>[2x]MTYTTRQIGAKNTLEYKVYIEKDGKPVSAFHDIPLYADKENNIFNMVVEIPRWTNAKLEITKEETLNPIIQDTKKGKLRFVRNCFPHHGYIHNYGAFPQTWEDPNVSHPETKAVGDNDPIDVLEIGETIAYTGQVKQVKALGIMALLDEGETDWKVIAIDINDPLAPKLNDIEDVEKYFPGLLRATNEWFRIYKIPDGKPENQFAFSGEAKNKKYALDIIKETHDSWKQLIAGKSSDSKGIDLTN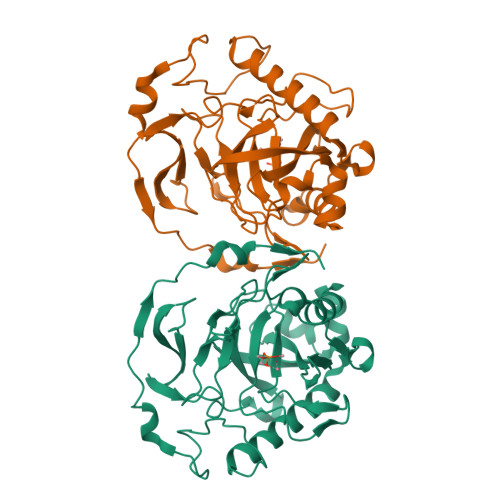VTLPDTPTYSKAASDAIPPASPKADAPIDKSIDKWFFISGSV> MGEIVSNEKSGVCINAPAKTKLQPSVFHQVFEGSKEPAVLNSKDPRLKTDFEEAIFSKYTGNKIMLMDEYMEEAVDHYVGCLEPLDISVDPIPLESAMYGMDGLEALDLTTSAGFPYLLQGKKKRDIFNRHTRDTTEMTKMLEKYGVDLPFVTFVKDELRSKEKVEKGKSRLIEASSLNDSVAMRVAFGNLYATFHSNPGTATGSAVGCDPDIFWSKIPILLDGEIFAFDYTGYDASLSPVWFACLKKVLIKLGYTHQTSFIDYLCHSVHLYKDRKYIVNGGMPSGSSGTSIFNTMINNIIIRTLLIRVYKGIDLDQFKMIAYG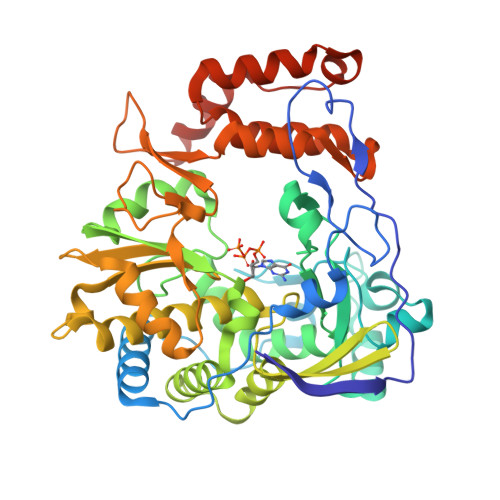DDVIASYPHKIDPALLAEAGKHYGLVMTPADKGTSFVDTNWENVTFLKRYFRADDQYPFLIHPVMPMKEIHESIRWTKDPRNTQDHVRSLCYLAWHNGEEAYNEFCRKIRSVPVGRALTLPAYSSLRRKWLDSFGSSGHHHHHH>PMFIVNTNVPRASVPDGFLSELTQQLAQATGKPPQYIAVHVVPDQLMAFGGSSEPCALCSLHSIGKIGGAQNR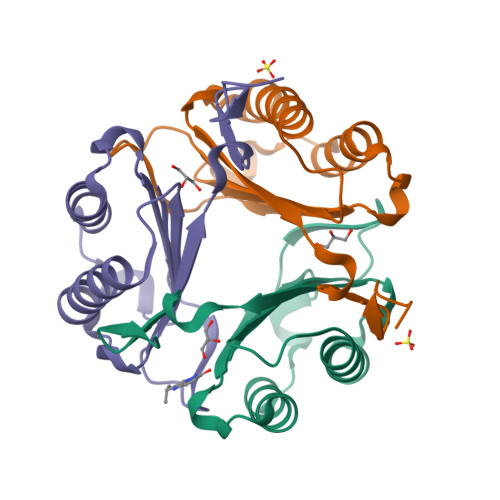SYSKLLCGLLAERLRISPDRVYINYYDMNAANVGWNNSTFALEHHHHHH[3x]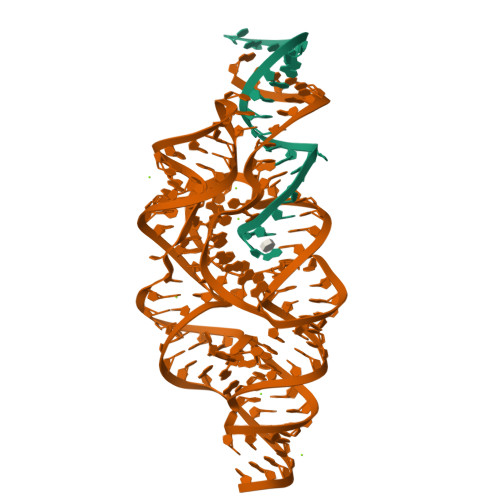> AGCGCCUGGACUUAAAGCCAUUGCACU;> CCGGCUUUAAGUUGACGAGGGCAGGGUUUAUCGAGACAUCGGCGGGUGCCCUGCGGUCUUCCUGCGACCGUUAGAGGACUGGUAAAACCACAGGCGACUGUGGCAUAGAGCAGUCCGGGCAGGAA>MTVRVAINGFGRIGRNVVRALYESGRRAEITVVAINELADAAGMAHLLKYDTSHGRFAWEVRQERDQLFVGDDAIRVLHERSLQSLPWRELGVDVVLDCTGVYGSREHGEAHIAAGAKKVLFSHPGSNDLDATVVYGVNQDQLRAEHRIVSNASATTNSIIPVIKLLDDAYGIESGTVTTIHSAMHDQQVIDAYHPDLRRTRAASQSIIPVDTKLAAGITRFFPQFNDRFEAIAVRVPTINVTAIDLSVTVKKPVKANEVNLLLQKAA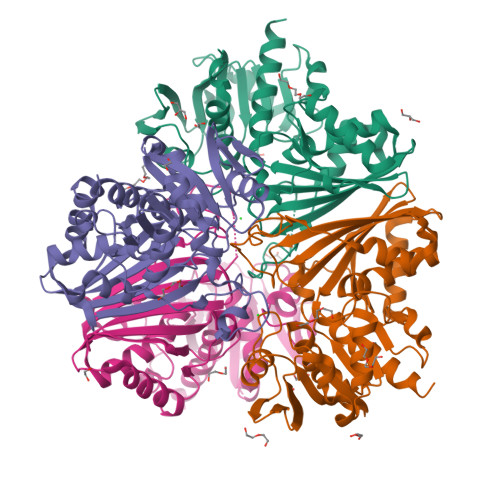QGAFHGIVDYTELPLVSVDFNHDPHSAIVDGTQTRVSGAHLIKTLVWCDNEWGFANRMLDTTLAMATVAFR[4x]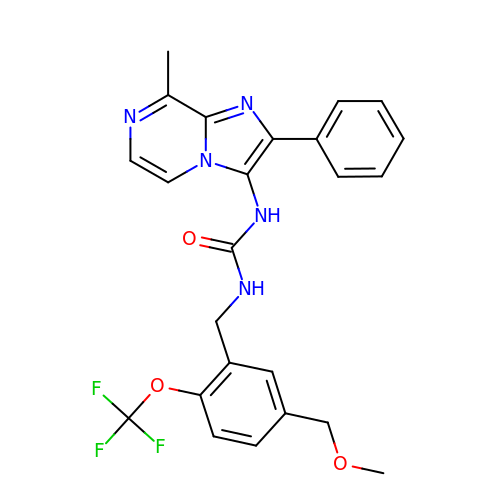N-{[5-(methoxymethyl)-2-(trifluoromethoxy)phenyl]methyl}-N'-(8-methyl-2-phenylimidazo[1,2-a]pyrazin-3-yl)urea | C24 H22 F3 N5 O3 | KNZNJSNITSGMNY-UHFFFAOYSA-N>MAKKTSSKGKLPPGPTPLPFIGNYLQLNTEQMYNSLMKISERYGPVFTIHLGPRRVVVLCGHDAVREALVDQAEEFSGRGEQATFDWVFKGYGVVFSNGERAKQLRRFSIATLRDFGVGKRGIEERIQEEAGFLIDALRGTGGANIDPTFFLSRTVSNVISSIVFGDRFDYKDKEFLSLLRMMLGIFQFTSTSTGQLYEMFSSVMKHLPGPQQQAFQLLQGLEDFIAKKVEHNQRTLDPNSPRDFIDSFLIRMQEEEKNPNTEFYLKNLVMTTLQLFVGGTETVSTTLRYGFLLLMKHPEVEAKVHEEIDRVIGKNRQPKFEDRAKMPYMEAVIHEIQRFGDVIPMSLARRVKKDTKFRDFFLPKGTEV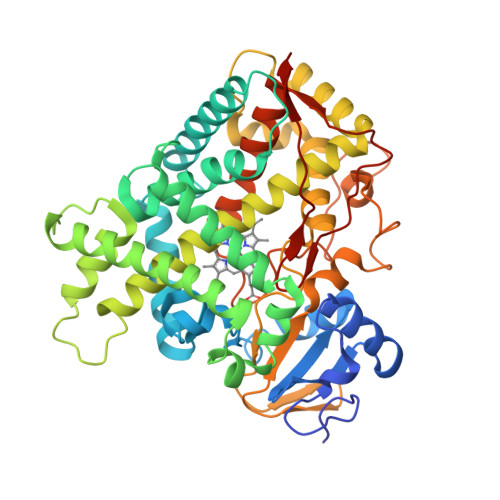YPMLGSVLRDPSFFSNPQDFNPQHFLNEKGQFKKSDAFVPFSIGKRNCFGEGLARMELFLFFTTVMQNFRLKSSQSPKDIDVSPKHVGFATIPRNYTMSFLPRHHHH[4x]N-{(2S)-3-[(R)-[(1R)-1-amino-2-phenylethyl](hydroxy)phosphoryl]-2-benzylpropanoyl}-L-phenylalanine 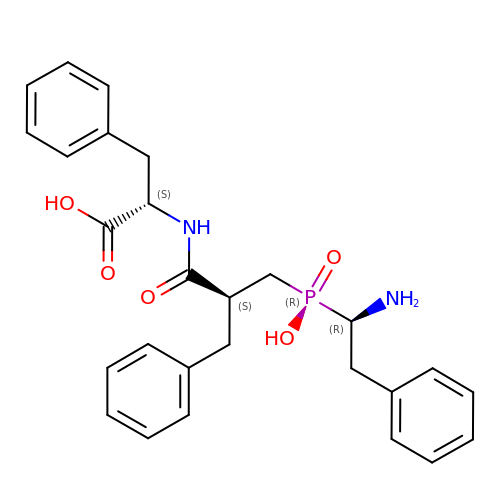| C27 H31 N2 O5 P | XNPYGVCNHOXQRJ-DSNGMDLFSA-N> GAMGTAQSKRSLWDFASPGYTFHGLHRAQDYR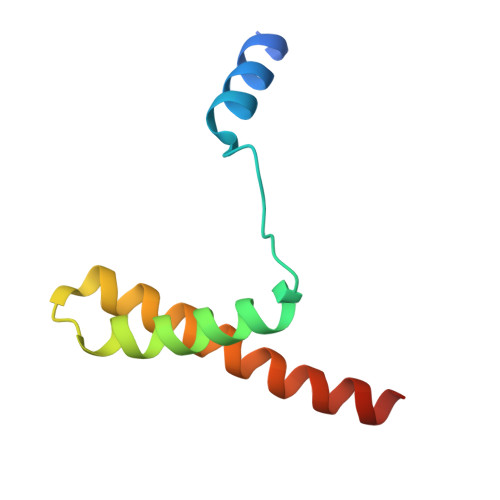RELDTLQSLLTTSQSSELQAAAALLKCQQDDDRLLQIILNLLHKV> MENLVGLLRIHVKRGVNLAIRDISSSDPYI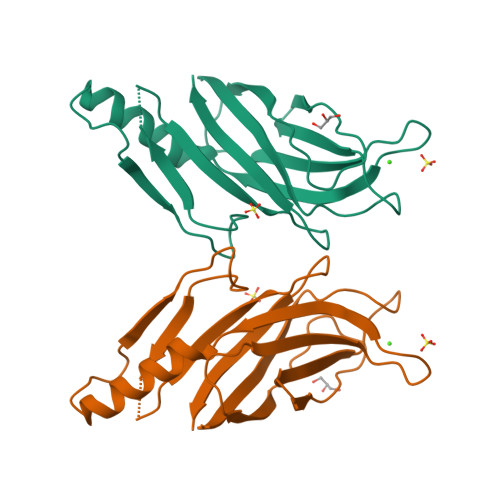VVHCGKQKLKTRVVKHSVNPEWNDDLTLSVTDPNLPIKLTVYDYDLLSADDKMGEAEFHIGPFIEAIKFAHQLGPGLPNGTIIKKIEPSRKNCLSESSHIVLNQGKIVQNMFLRLQHVECGEVELQLEWIDVPGSRGI> YASRTKVFPGERVEHVTFNFTLENQIHRGGQYFNDKFIGLRLKSVSFEDSLFEECYFEDVTSSNTFFRNCTFINTVFYNTDLFEYKFVNSRLINSTFLHNKEGCPLDV;> KNIVNTSILSIVYKKDDLIDLSRYGAKINIGDRVYYDSIDKNQIKLINLESSTIEVILKNAIVYNSMYENFSTSFWIKIPKYFSKINLNNEYTIINCIENNSGWKVSLNYGEIIWTLQDNKQNIQRVVFKYSQMVNISDYINRWIFVTITNNRLTKSKIYINGRLIDQKPISNLGNIHASNKIMFKLDGCRDPRRYIMIKYFNLFDKELNEKEIKDLYDSQSNSGILKDFWGNYLQYDKPYYMLNLFDPNKYVDVNNIGIRGYMYLKGPRGSVVTTNIYLNSTLYEGTKFIIKKYASGNEDNIVRNNDRVYINVVVKNKEYRLATNASQAGVEKILSALEIPDVGNLSQVVVMKSKDDQGIRNKCKMNLQDNNGNDIGFIGFHLYDNIAKLVASNWYNRQVGKASRTFGCSWEFIPVDDGWGESSL

Synaptic vesicle glycoprotein 2a (SV2A), a putative membrane transporter in the synaptic vesicles (SVs), has been identified as a target of LEV and BRV. SV2A also serves as a receptor for botulinum neurotoxin (BoNT), which is the most toxic protein and has paradoxically emerged as a potent reagent for therapeutic and cosmetic applications. SV2 family proteins belong to the major facilitator superfamily (MFS) with 12 predicted transmembrane helices. In addition to the transmembrane domain (TMD) core, a cytosolic N-terminal region and a large fourth luminal domain (LD4) are present.

The quality of the cryo-EM map is sufficient for modeling the SV2A and HCA2, except that the peripheral region of the HCA2 shows poor density. Additional masked local refinement improved the map quality covering HCA2 and SV2A LD4 (LD4A). Masked local refinement revealed the well-ordered densities of the N-glycans at the binding interface. The open edge of the β-strand from the β-hairpin of HCA2 forms backbone hydrogen bonding interactions with the open edge of the C-terminal β-strand from the β-helix structure of LD4A. In addition to the backbone–backbone interaction, the SV2A His578 side chain forms a salt bridge with the BoNT/A2 Glu1156 side chain. SV2A Phe576 contributes to the van der Waals interactions with Ser1142 and Val1144 of BoNT/A2. The protein–protein interaction between HCA2 and LD4A creates a relatively small binding interface with a buried surface area of 464 Å2. To enhance this interaction, N-glycans attached to LD4A contribute to binding. A N-glycan containing two N-acetylglucosamines (NAG)s and fucose (FUC) attached to Asn573 forms extensive contacts with HCA2. The BoNT/A2 Phe953 and the aliphatic portion of the BoNT/A2 Arg1064 form the van der Waals contacts with the two NAGs attached to LD4A.>[2x]MGHHHHHHMDMTKIALLSDIHGNTTALEAVLADARQLGVDEYWLLGDILMPGTGRRRILDLLDQLPITARVLGNWEDSLWHGVRKELDSTRPSQRYLLRQCQYVLEEISLEEIEVLHNQ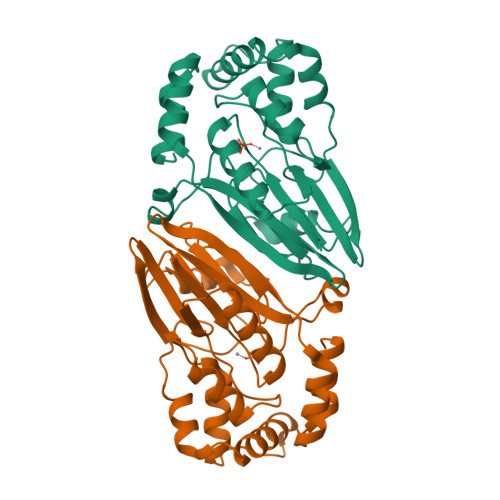PLQIHRQFGDLTVGISHHLPDKNWGRELIHTGKQEEFDRLVTHPPCDIAVYGHIHQQLLRYGTGGQLIVNPGSIGQPFFLDAQLRKDLRAQYMILEFDDKGLVDMDFRRVDYDVAAELQLAKDLRLPYFEVYYESLVNGIHHTHHQEFLRE> MKEFYLTVEQIGDSIFERYIDSNGRERTREVEYKPSLFAHCPESQATKYFDIYGKPCTRKLFANMRDASQWIKRMEDIGLEALGMDDFKLAYLSDTYNYEIKYDHTKIRVANFDIEVTSPDGFPEPSQAKHPIDAITHYDSIDDRFYVFDLLNSPYGNVEEWSIEIAAKLQEQGGDEVPSEIIDKIIYMPFDNEKELLMEYLNFWQQKTPVILT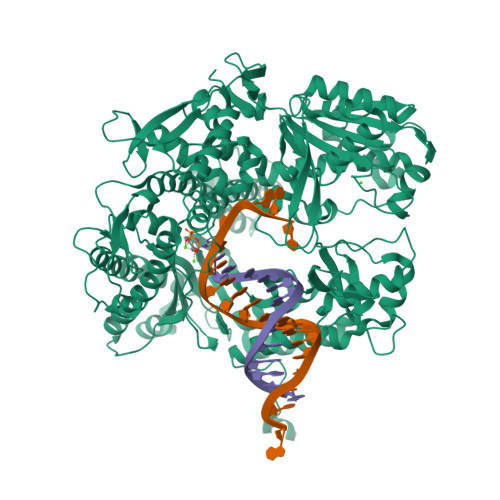GWNVESFAIPYVYNRIKNIFGESTAKRLSPHRKTRVKVIENMYGSREIITLFGISVLDYIDLYKKFSFTNQPSYSLDYISEFELNVGKLKYDGPISKLRESNHQRYISYNIIAVYRVLQIDAKRQFINLSLDMGYYAKIQIQSVFSPIKTWDAIIFNSLKEQNKVIPQGRSHPVQPYPGAFVKEPIPNRYKYVMSFDLTSAYPSIIRQVNISPETIAGTFKVAPLHDYINAVAERPSDVYSCSPNGMMYYKDRDGVVPTEITKVFNQRKEHKGYMLAAQRNGEIIKEALHNPNLSVDEPLDVDYRFDFSDEIKEKIKKLSAKSLNEMLFRAQRTEVAGMTAQINRKALINGLAGALGNVWFRYYDLRNATAITTFGQMALQWIERKVNEYLNEVCGTEGEAFVLYGDTDSIYVSADKIIDKVGESKFRDTNHWVDFLDKFARERMEPAIDRGFREMCEYMNNKQHLMFMDREAIAGPPLGSKGIGGFWTGKKRYALNVWDMEGTRYAEPKLKIMGLETQKSSTPKAVQKALKECIRRMLQEGEESLQEYFKEFEKEFRQLNYISIASVSSANNIAKYDVGGFPGPKCPFHIRGILTYNRAIKGNIDAPQVVEGEKVYVLPLREGNPFGDKCIAWPSGTEITDLIKDDVLHWMDYTVLLEKTFIKPLEGFTSAAKLDYEKKASLFDMFDF> MSLADTRKIDSVLLIDDDDIVNFLNT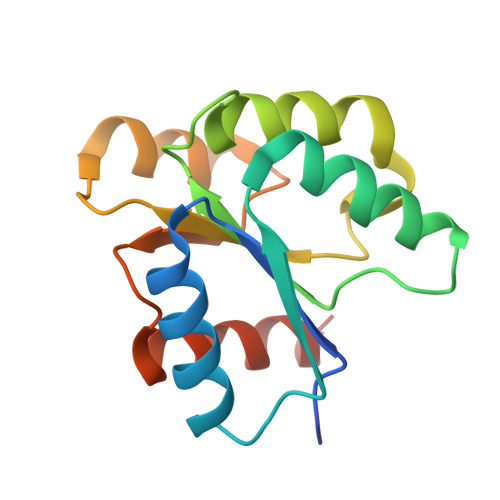TIIRMTHRVEEIQSVTSGNAAINKLNELYAAGRWPSIICIDINMPGINGWELIDLFKQHFQPMKNKSIVCLLSSSLDPRDQAKAEASDWVDYYVSKPLTANALNNLYNKVLNEGHHHHHH TWIK1 (K2P1.1, KCNK1) is a widely expressed pH-gated two-pore domain K+ channel (K2P) that contributes to cardiac rhythm generation and insulin release from pancreatic beta cells. K2Ps assemble as homo- or hetero-dimers, with each subunit containing four transmembrane-spanning helices (TM1–TM4), two selectivity filters (SF1–SF2), two pore helices (PH1–PH2), and two extracellular cap helices (CH1–CH2). TWIK1 is a pH-gated K+ channel that responds to extracellular acidification. To capture structures of TWIK1 in open and closed states within a lipid environment, we reconstituted the channel in nanodiscs containing the lipids DOPE, POPC, and POPS and determined its structure by cryo-EM at pH 7.4 and pH 5.5 to ~3.4 Å resolution.

At high pH, TWIK1 adopts an open conformation. The high pH structure shows an unobstructed path from the intracellular to extracellular solutions through the channel cavity, selectivity filter, and bifurcated extracellular tunnels under the helical cap. At high pH, the selectivity filter adopts a nearly four-fold symmetric conformation with K+ ions bound at five positions in sites S0-S4, as observed in other conductive K+ channels and the previously reported TWIK1 crystal structure at pH 8 (Cα r.m.s.d. within pore helices and selectivity filters = 0.6 Å). At high pH, the residues immediately after the selectivity filter, H122 and D230, project back behind the filter and away from the conduction axis. At high pH, a wide-open path ~3 Å in radius leads from the extracellular solution to the selectivity filter above H122 and D230 and below CH2s. The constriction in the lateral membrane opening at high pH is slightly smaller than the cross-section of an acyl-chain methylene (12.6 Å) and, consistently, similar acyl chain density is not observed in the TWIK cavity at high pH. The TWIK1 lateral membrane opening at high pH is larger than that observed in other conductive K2P structures, including TRAAK and TASK2, and just small enough to prevent lipid acyl chain access to the cavity. While the conformation we observe at high pH is likely predominant under these conditions, we cannot exclude the existence of a subpopulation of particles with a slightly larger opening containing cavity bound acyl chains. The high pH reconstruction is more anisotropic due to preferred orientations of particles. Some regions, particularly the intracellular termini and TM2–TM3 linker, are less well resolved in the high pH map, but amino acids G24 to F280 could still be confidently modeled.

>[2x]MLQSLAGSSCVRLVERHRSAWCFGFLVLGYLLYLVFGAVVFSSVELPYEDLLRQELRKLKRRFLEEHECLSEPQLEQFLGRVLEASNYGVSVLSNASGNWNWDFTSALFFASTVLSTTGYGHTVPLSDGGKAFCIIYSVIGIPFTLLFLTAVVQRVTVHVTRRPVLYFHIRWGFSKQVVAIVHAVLLGFVTVSCFFFIPAAVFSVLEDDWNFLESFYFCFISLSTIGLGDYVPGEGYNQKFRELYKIGITCYLLLGLIAMLVVLETFCELHELKKFRKMFYVKKDKDEDQVHIMEHDQLSFSSITEQAAGLKEEQKQNEPFVASQSPPYEDGSANH4-(3-ethylthiophen-2-yl)benzene-1,2-diol | C12 H12 O2 S | 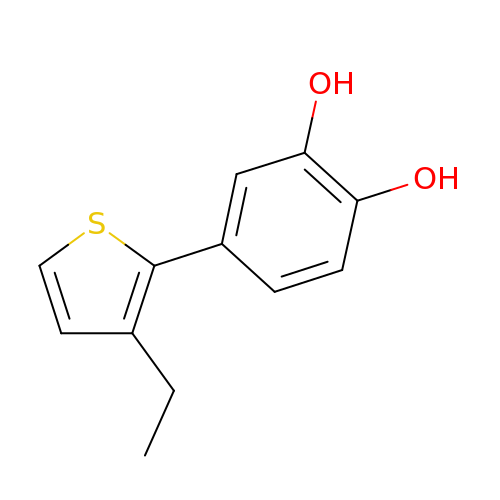VXLXQOMDQVQQLA-UHFFFAOYSA-N> GSSSGGSGHTPTTQATHADDHDLTTHNGTEEHDDGHDDGHDDLHAHAPKVIVFISGSCLFGAISRSLFKKLPIPYTVVLLILGAILGVVASNVPLVEEHTRDVAHMDPHVLLQIFLPVLIFESAFAMDVHTFMRSFSQVCILALFGLVVASVLTAVLAMNLFNYNWNFSEAMMFGAIMSATDPVAVVALLKDLGASKQLGTIIEGESLLNDGCAIVIFNVFMKMVFFPQLTSTVGQNVLYFLQVAVAGPLWGYAVAKVTVFFLSH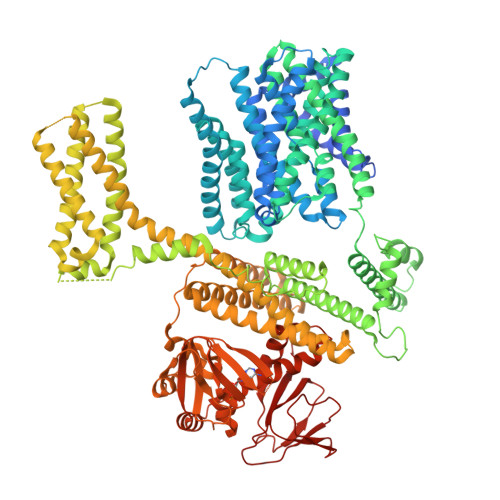IFNDALVEITITLAATYLTYYIGDIWLEVSGVLAVVVLGLIVNAEKTSISPEVEVFLHRFWEMLAYLANTLIFMMVGVVVTQKALVAVDKMDWFYLIILYLAITIIRGMVISLFSPILSRIGYGLTWRNAVIMTWGGLRGAVGLALALVVENLAGNDVIGSKFLFHTAGIVVLTLVINATTIQTLLRILGMSDISIPKRLAMAGAVRRIHEGQNRTLNMLKSDRFLADADWDIATAACEISDPYSALSDDENAPADELTLGERKSVCPGCKAMVPNEPSPREFADMMEEARLRMLKAEKISYWKQFEHGMLAREALRLLVQHAEVAADEKDQFILVDDLKKSWQIKGIYPWLKRKLEDLISEKKIAAIPMPKYKLGKLMYKICHHMAFEVTINIAIVLNIVPIIMEFVVQDKMASVSTMAAPGSTVSSEPSSLQKIEDALRISNYVFFVIYAIEAIVKILGLGRHYIVSHWNKFDAFILVVALVDIIIAETLLKGSITINLSSIKVVKLFRLLRGLRMLRLTKALIPKLILVVNGKINNQLSLGYDVGKGYIIGEEEVGKIIDRMVDNKKILRELKHISETGRLQVVKELGLLQREHPGIAVSVKTRQAIRTILNHSRETIHELQGAGLLDEMEAHKLELTVEIKMKRLMNAPSSIPPPPPENLLKNVSWLAGDMKLIDFIKARASLLHFDYGEVIVREGDESDGLFLIVSGLVKLYGKSAFLDHDNPPVTAGSEENEVFEDYLTVGNVIGEMGVLTKKPRNATVTCETTVQVYFITAEDMNIAIDTFTLYPSLEYRLWRVVAIRIATPLIMEQMAFQGWTQEKVKLHLERGYLVDLAESHFQFNIDATLEDVILINGTAYNAHTREEIRSPCLISRTVHKLTFQYTATEEPRLFVVRNAEY>[4x]SNAMSEPLHALARQL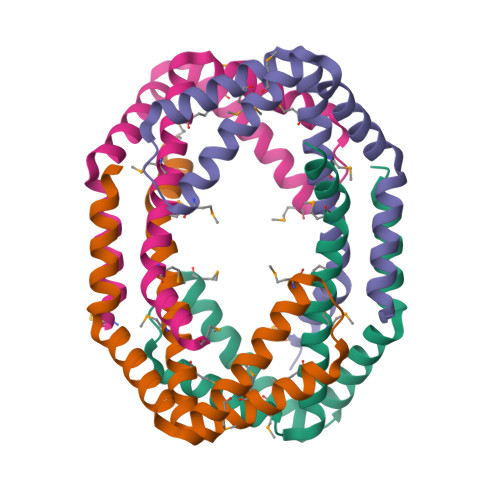EQAIRASEPFQQLKRAYEDVRRDETAYRMFANVRDIQLRLHEKQMRGAAILPDEIEQAQKAMALAQQNEKLARLMALEQQMSITIAEVQQIAMKPLEELHRSFMEGR>[4x]DHYNCVSSGGQCLYSAC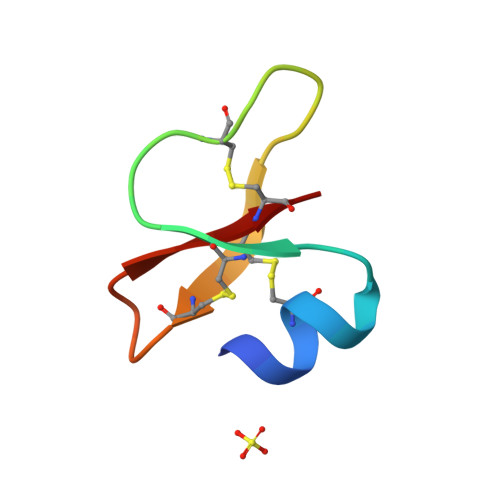PIFTKIQGTCYRGAAKCCK>AQCSVDIQGNDQMQFNTNAITVDKSCKQFTVNLSHPGNLPKNVMGHNWVLST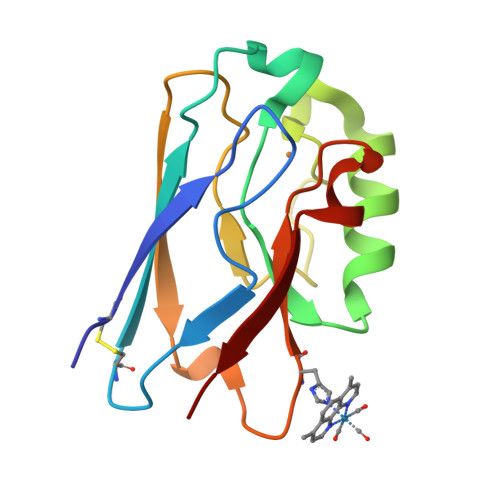AADMQGVVTDGMASGLDKDYLKPDDSRVIAQTKLIGSGEKDSVTFDVSKLKEGEHYMFFCTFPGHSALMKGTLTLK[2x]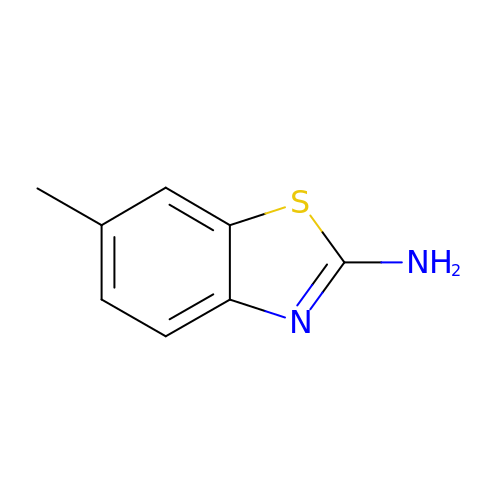6-methyl-1,3-benzothiazol-2-amine | C8 H8 N2 S | DZWTXWPRWRLHIL-UHFFFAOYSA-N> GSHMSLIKDQMTTKLHLEGTVNGHYFEIEGNGQGEPYEGKQSMKLVVTKGAPLPFAYDILLPQHMYGSKPFIKYPAEIPDYYKQSFPEGFSWERIMKFEDGA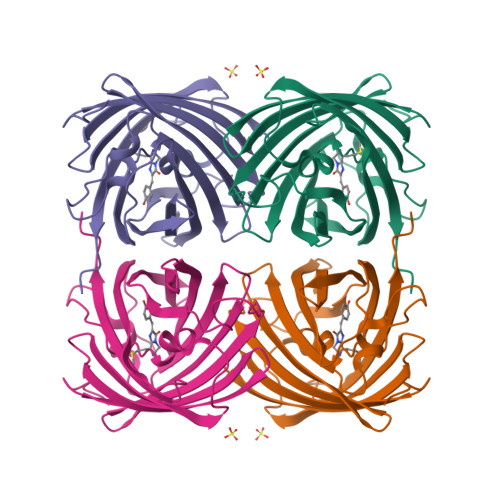VCTVSQHSSLKGNCFVYDVKFHGVHFPLDGPVMQKKTLGWEPSTERIYPRDGMLRGDVPMALKVEGGGNYRCDFKTVYKAKKSVKLPENHFVDHRIVMTKHDKDYTNVEQAEVAVARNSPF21-hydroxy-oligomycin | C45 H74 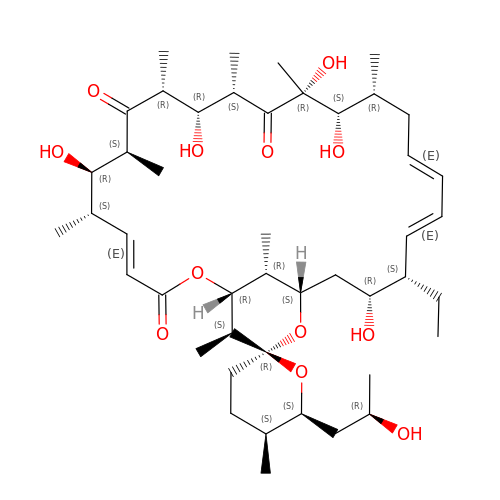O12 | SCVGLVGTMYJVOI-AAYFJTACSA-N>VVGGVNAEKGAWPWMVSLHWRGRHGCGASLIGRDWLLTAAHCVYGKNTHLQYWSAVLGLHAQSSMNSQEVQIRQVDRIIINKNYNRRTKEADIAMMHLQQPVNFTEWVLPVCLASEDQHFPAGRRCFIAGWGRDAEGGSLPDILQEAEVPLVDQDECQRLLPEYTFTSSMLCAGYPEGGVDSCQGDSGGPLMCLEDARWTLIGVTSFGVGCGRPERPGAYARVSAFTSWIAETRR[2x]

Because of the unique specificity, enteropeptidase could be used as a tool for the production of recombinant fusion proteins. Especially the recombinant enteropeptidase light chain (EPL), which contains a catalytic domain, is of large interest to be applied in biopharmaceutical industry. Recently, the enteropeptidase from medaka had been reported to be a more effective tool, because of its much stricter specific for the D4K sequence compared to its mammalian counterparts. Therefore, we sought to solve the crystal structure of the light chain of medaka enteropeptidase (MEPL), and gain insights into the determinants for its stricter specificity.

The structure of MEPL displays a typical α/β trypsin—like serine protease fold. It consists of two six-stranded β-barrels (β1–β6 and β7–β12), either of which makes up about one half of the entire molecule. Superimposing of MEPL with the bovine enteropeptidase light chain resulted in an rmsd of 0.79 Å for the Ca coordinates. The differences are mainly located in the loop regions, such as the so-called ‘131-loop’ that connects strand β7 and β8. MEPL also contains, relative to bovine enzyme, an additional small 310-helix between the strand β4 and β5. Compared with BEPL and HEPL, MEPL shows much less activity for the peptide substrates with arginine at P1 site, which indicates its restriction for the entrance of arginine residues. In MEPL structure, MEPLE136 makes three hydrogen bonds with MEPLR213, while there are no similar interactions in BEPL because it is BEPLL213, BEPLY136 in these positions as well as the same situation for the HEPL structure. In addition, MEPLV209 and MEPLG210 with short side chains are covered and fixed by the side chains of four residues (MEPLE136, MEPLE163, MEPLR213 and MEPLR216), reducing the mobility of “208-loop” and strand β11 in MEPL. Moreover, we observed that the imidazole group of MEPLH24 could form a hydrogen bond with the main chain oxygen atom of MEPLG185, which could help improving the structural rigidity of “174-loop”. Over all, the unique residue interactions in MEPL may reduce the flexibility of the specific pocket, restricting the entrance of arginine residue which has larger side chain.>MDFKYTEEKETIKINNIMIHKYTVLYTSNCIMDIYSEEEKITCFSNRLVFLERGVNISVRMQKQILSEKPYVAFRLNGDMLRHLKDALMIIYGMSKIDTNACRSMSRKIMTTEVNKTLLDELKNINSHDNSAFISSLIYLISKLENNEKIIESIYISSVSFFSDKVRNLIEKDLSRKWTLGIIADAFNASEITIRKRLESENTNFNQILMQLRMSKAALLLLENSYQISQISNMIGISSASYFIRIFNKHYGVTPKQFFTYFKGG[2x]

While ETEC colonization factors are diverse, nearly half are regulated by the transcription factor Rns (also known as CfaD or CfaR), a member of the AraC family. Rns activates pili loci expression by binding to a site immediately adjacent to the -35 hexamer, which may be accompanied by one or more additional sites further upstream. Rns shows the typical characteristics of two-domain AraC family proteins. The DNA binding domain (DBD) (residues 162–265) consists of seven alpha helices linked to the N-terminal domain by a 3 residue linker.

Given decanoic acid both stabilized and affected Rns function, we crystalized it in the presence of excess decanoic acid, ensuring saturation, to assess what effects this might have on its structure. Despite the diffraction data showing significant pseudo-translation, the structure was solved to 3.0 Å using molecular replacement with the apo SeMet-Rns structure as a search model. Analysis of the resulting electron density showed both monomers contained electron density consistent with a ligand, which we again modeled as decanoic acid. In the unlabeled structure both monomers in the ASU were in the closed conformation. Therefore, we examined differences between the open monomer observed in the SeMet structure and a closed monomer of the unlabeled structure. The two conformations were aligned using the long helix in the DBD. This highlighted that helices making up the dimer interface and β-strands 2, 4, and 6 in the open conformation are shifted away from the long helix in the DBD by ~ 1.7 Å in comparison to the closed conformation. In both the open and closed conformations, His20 and Arg75 interact with the carboxyl group of the decanoic acid. In the open structure, Arg75 is between the fatty acid and the rest of the N-terminal domain, whereas in the closed structure, Arg75 is more alongside the ligand. In the closed conformation the fatty acid carboxyl group is turned 90° allowing both oxygens to make contacts with either His20 or Arg75.> SMGWLHPNDKVMGPGVSY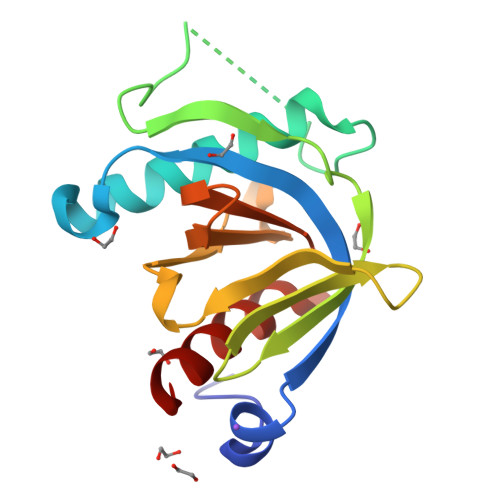LVRYMGCVEVLQSMRALDFNTRTQVTREAISLVCEAVPGAKGATRRRKPCSRPLSSILGRSNLKFAGMPITLTVSTSSLNLMAADCKQIIANHHMQSISFASGGDPDTAEYVAYVAKDPVNQRACHILECPEGLAQDVISTIGQAFELR>MDEFEMIKRNTSEIISEEELREVLKKDEKSALIGFEPSGKIHLGHYLQIKKMIDLQNAGFDIIIILADLHAYLNQKGELDEIRKIGDYNKKVFEAMGLKAKYVYGSEFMLDKDYTLNVYRLALKTTLKRARRSMELIAREDENPKVAEVIYPIMQVNGIHYVGGDVAVGGMEQRKIHMLARELLPKKVVCIHNPVLTGL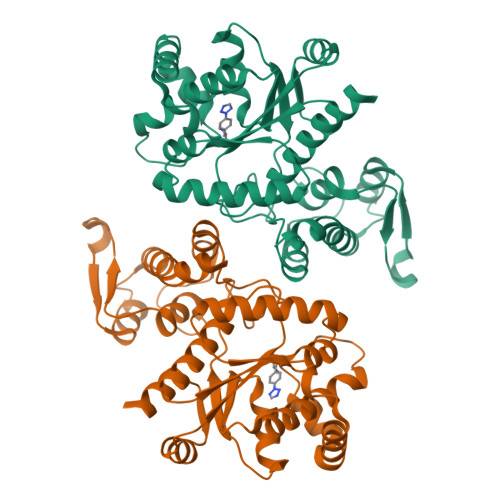DGEGKMSSSKGNFIAVDDSPEEIRAKIKKAYCPAGVVEGNPIMEIAKYFLEYPLTIKRPEKFGGDLTVNSYEELESLFKNKELHPMDLKNAVAEELIKILEPIRKRLLEHHHHHH[2x]Diphosphonucleotide phosphatase/phosphodiesterase (PPD1), a glycoprotein plant purple acid phosphatase (PAP) from yellow lupin seeds, contains a bimetallic Fe–Mn catalytic site which is most active at acidic pH. Unlike other plant PAPs, PPD1 cleaves the pyrophosphate bond in diphosphonucleotides and the phosphodiester bond in various phosphodiesters. Purple acid phosphatases (PAPs; EC 3.1.3.2) catalyze the hydrolysis of inorganic phosphorus from a broad range of phosphate monoesters and anhydrides in the pH range 4–7. PAPs are acidic metallohydrolases with the metal centre comprising an iron(III) ion and a divalent metal, which is either a zinc(II), manganese(II) or iron(II) ion.

The homohexameric organization of PPD1, as revealed by a 1.65 Å resolution crystal structure and confirmed by solution X-ray scattering, is unique among plant PAPs, for which only homodimers have previously been reported. The overall structure of the PPD1 subunit is defined by two domains: a sweet potato-like PAP domain, containing the Fe–Mn active site, and a previously uncharacterized N-terminal domain with unknown function. The N-terminal domain (residues 1–150) of PPD1 consists primarily of two β-sheets making up a seven-stranded β-­barrel. A 26-residue loop (Phe59–Pro85) joining β-strands 3 and 4 extends about 20 Å from the barrel and into the active-site solvent channel of the PAP domain. This extension positions the Lys74 side chain on the loop 10 Å from the phosphate-binding site and 8 Å from the Ser589 residue of the neighbouring subunit. Five disulfide bridges are present within each subunit, three of which are involved in positioning the structural elements that form the trimer interfaces. The solvent-accessible C-terminal end of each subunit (residues 583–589) is oriented by the Cys577–Cys582 bridge so that it traverses the adjoining subunit, protruding into its Fe–Mn active site and placing the side chain of the terminal Ser589 within 8 Å of the two metal atoms. Analysis of the crystal structure of PPD1 using the PDBePISA server suggests that its most probable quartenary structure is a hexamer, with an estimated dissociation free energy of 42 kcal mol−1 compared with 24 kcal mol−1 for the trimer. Previously, we identified an Fe–Mn bimetallic centre in PPD1, examined its oxidation state and demonstrated that it requires iron and divalent metal for its enzymatic activity. The crystal structure shows the active site of PPD1 with a phosphate ion bound to both of the metal atoms, similar to that previously described to be unique for sweet potato PAP. The Mn atom is coordinated by His434, His476, Asn345 and the bridging Asp312.

>[3x]DEHAYIKATPNVLGFEGHYTEWVTLQYSNNKPSIDDWIGVFSPANFSASTCPGENKMTNPPFLCSAPIKFQYANFSSHSYKDTGKGSLKLQLINQRSDFSFALFTGGLTNPKLIAVSNKVSFVNPNAPVYPRLAQGKTWDEITVTWTSGYDINDAEPFVEWGPKEGNLVKTPAGTLTFDRNTMCGAPARTVGWRDPGYIHTSFLKELWPNREYTYKLGHRLFNGTTIWSKEYHFKASPYPGQSSVQRVVIFGDMGKAEADGSNEYNNFQPGSLNTTKQIIQDLEDIDIVFHIGDLCYANGYISQWDQFTAQIEPIASTVPYMTASGNHERDWPGTGSFYGNLDSGGECGVPAQTMFFVPAENREKFWYSTDYGMFRFCIAHTELDWRKGTEQYEFIEKCLASVDRQKQPWLIFLAHRVLGYSSAGFYVQEGSFEEPMGREDLQHLWQKYKVDIAMYGHVHNYERTCPIYQNVCTNKEKHNYKGNLNGTIHVVVGGGGASLAEFAPINTTWSIFKDHDFGFVKLTAFDHSNLLLEYRKSSDGQVYDSFTISRDYRDILACSVDSCPTTTLAS> IVGGYTCGANTVPYQVSLNSGYHFCGGSLINSQWVVSAAHCYKSGIQVRLGEDNINVVEGNEQFISASKSIVHPSYNSNTLNNDIMLIKLKSAASLNSRVASISLPTSCASA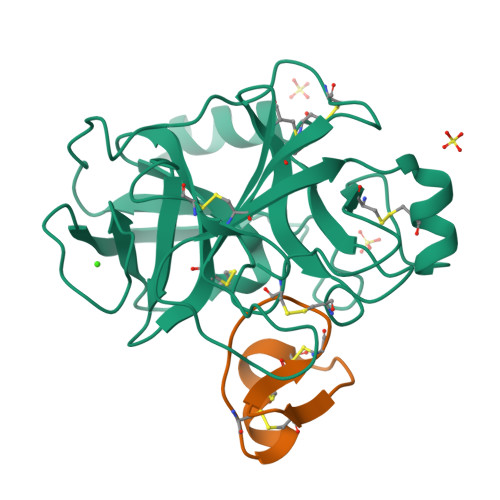GTQCLISGWGNTKSSGTSYPDVLKCLKAPILSDSSCKSAYPGQITSNMFCAGYLEGGKDSCQGDSGGPVVCSGKLQGIVSWGSGCAQKNKPGVYTKVCNYVSWIKQTIASNCNYVSWIKQTIASN;> ILKRCKTYDDCKDVCKARKGKCEFGICKCMIK> GCPDGWTQFLDLCYIYQSAKA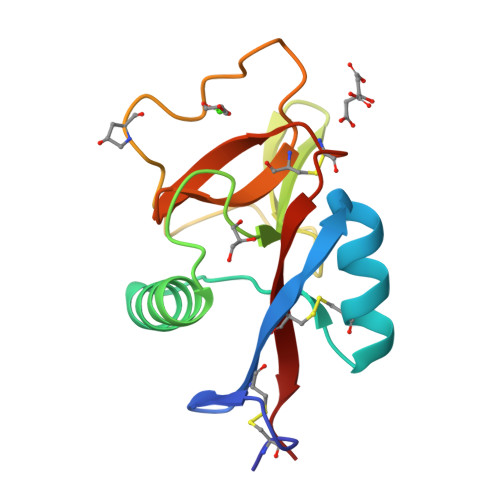SWASAQSSCQALGGILAEPDTACENEVLIHMCKENGDAGSFGPWLGGQKVGGAWQWSSSGAAFDYLRWGPNEPNNSGGNEDCLHYNWLSWNDLRCHYQASYLCQRAAE>[2x]HHHHHHGSMTKSALVTGASRGIGRSIALQLAEEGYNVAVNYAGSKEKAEAVVEEIKAKGVDSFAIQANVADADEVKAMIKEVVSQFGSLDVLVNNAGITRDNLLMRMKEQEWDDVIDTNLKGVFNCIQKATPQMLRQRSGAIINLSSVVGAV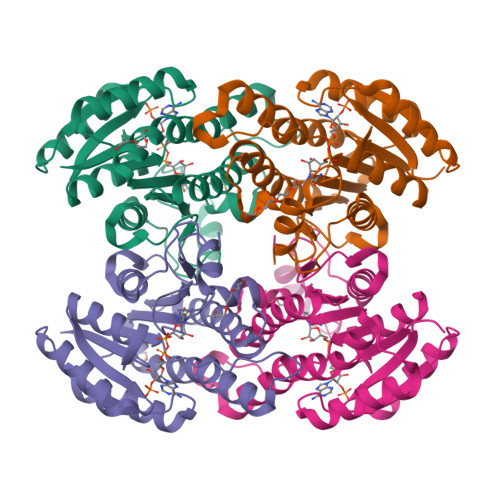GNPGQANYVATKAGVIGLTKSAARELASRGITVNAVAPGFIVSDMTDALSDELKEQMLTQIPLARFGQDTDIANTVAFLASDKAKYITGQTIHVNGGMYM>SMDHYKAKATRHIFLIRHSQYHVDGSLEKDRTLTPLGREQAELTGLRLASLGLKFNKIVHSSMTRAIETTDIISRHLPGVCKVSTDLLREGAPIEPDPPVSHWKPEAVQYYEDGARIEAAFRNYIHRADARQEEDSYEIFICHANVIRYIVCRAL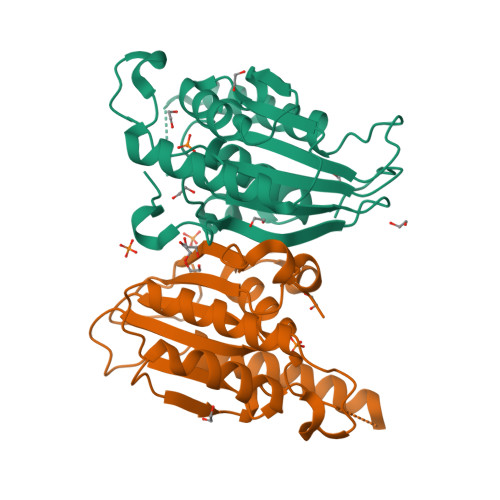QFPPEGWLRLSLNNGSITHLVIRPNGRVALRTLGDTGFMPPDKITRS[2x]> MASSRRESINPWTLTG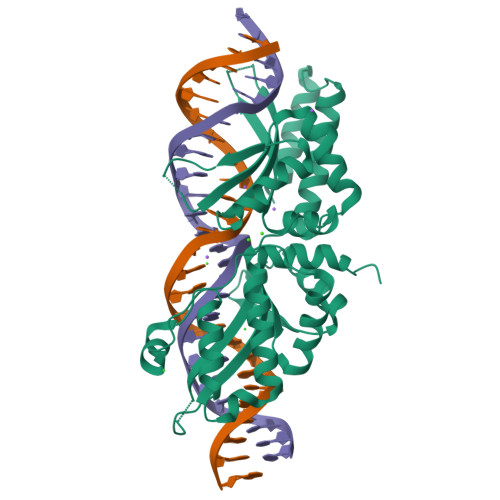FADAEGSFGLSILNRNRGTARYHTRLSFTIMLHNKDKSILENIQSTWKVGSILNNGDHYVSLVVYAFEDLKVIIDHFEKYPLITQKLGDYKLFKQAFSVMENKEHLKENGIKELVRIKAKMNWGLNDELKKAFPEVISRERPLINKNIPNGKWLAGFTSGDGSFFVRLRKSNVNARVRVQLVFEISQHIRDKNLMNSLITYLGCGHIYEGNKSERSWLQFRVEKFSDINDKIIPVFQENTLIGMKLEDFEDWCKVAKLIEEKKHLTESGLDEIKKIKLNMNKRR>[4x]TTSQKHRDFVAEPMGEKPVGSLAGIGEVLGKKLEERGFDKAYVVLGQFLVLKKDEDLFREWLKDTAGANAKQSRDAFGALREWADAFL;>[2x]SSFSQHARTSGRVAVEEVDEEGKFVRLRNKSNEDQSMGNWQIKRQNGDDPLLTYRFPPKFTLKAGQVVTIWAAGAGATHSPPTDLVWKAQNTWGCGNSLRTALINSTGEEVAMRKLVRS;>[2x]GDNYADLSDTEL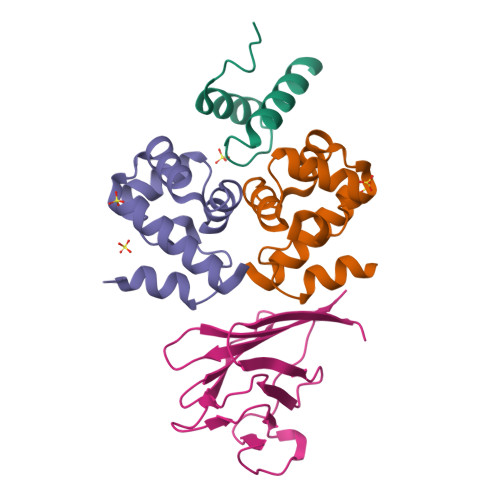TTLLRRYNIPHGPVVGSTRRLYEKKIFEYETQR N-[(2E)-3,7-dimethylocta-2,6-dien-1-yl]-L-glutamic 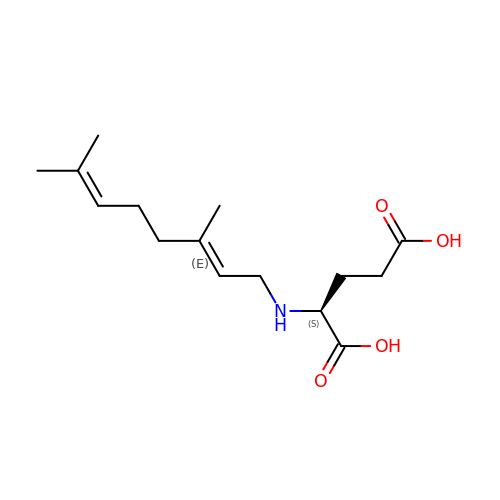acid | C15 H25 N O4 | WRAUYKHQSOIVEN-SRXBQZRASA-N>[2x]MHHHHHHMIEELGKIDRIIQESVPGKQITLAHVIAAPIEAVYECLGVDHEGAIGVVSLTPNETAIIAADIAGDAANIDICFVDRFTGSVMFSG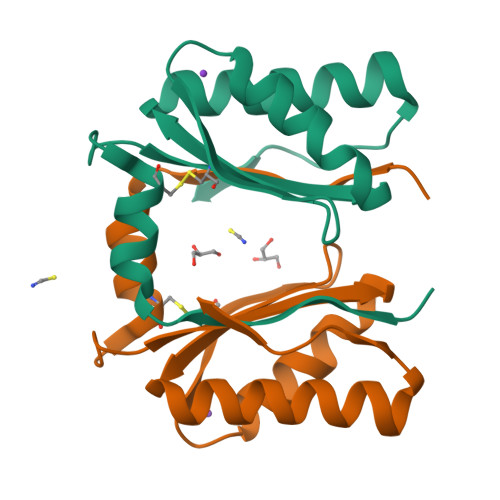DIQSVETSLEDILEYFKNSLGFSTVPLTKS CYTIDINE-5'-DIPHOSPHO-BETA-D-XYLOSE | C14 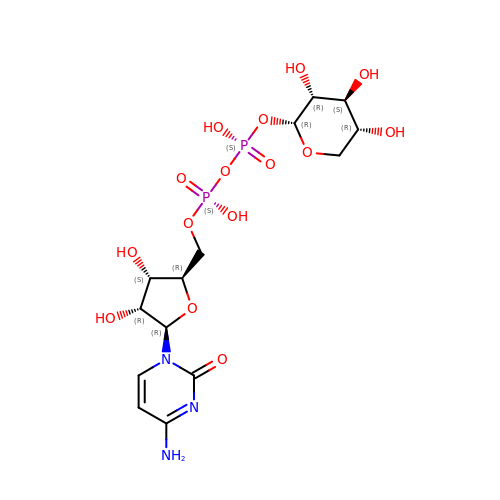H23 N3 O15 P2 | NWSKPSPTJOAICE-OCIMBMBZSA-N>VAQISPQYPMFTVPLPIPPVKQPRLTVTNPVNGQEIWYYEVEIKPFTHQVYPDLGSADLVGYDGMSPGPTFQVPRGVETVVRFINNAEAPNSVHLHGSFSRAAFDGWAEDITEPGSFKDYYYPNRQSARTLWYHDHAMHITAENAYRGQAGLYMLTDPAEDALNLPSGYGEFDIPMILTSKQYTANGNLVTTNGELNSFWGDVIHVNGQPWPFKNVEPRKYRFRFLDAAVSRSFGLYFADTDAIDTRLPFKVIASDSGLLEHPADTSLLYISMAERYEVVFDFSDYAGKTIELRNLGGSIGGIGTDTDYDNTDKVMRFVVADDTTQPDTSVVPANLRDVPFPSPTTNTPRQFRFGRTGPTWTINGVAFADVQNRLLANVPVGTVERWELINAGNGATHPIHIHLVDFKVISRTSGNNARTVMPYESGLKDVVWLGRRETVVVEAHYAPFPGVYMFHCHNLIHEDHDMMAAFNATVLPDYGYNATVFVDPMEELWQARPYELGEFQAQSGQFSVQAVTERIQTMAEYRPYAAADE[2x]

Bilirubin oxidase (MvBOx; EC 1.3.3.5) from the ascomycete plant pathogen Myrothecium verrucaria (Albifimbria verrucaria) is a member of the blue multicopper oxidase family (MCO). MCOs are capable of oxidizing various organic and/or inorganic substrates and reducing oxygen to water without release of reactive oxygen species. MvBOx, composed of 534 amino acid residues, consists of three cupredoxin-like domains with four copper ions forming two active sites. T1Cu is connected with the trinuclear cluster (TNC), composed of one type II (T2Cu) and two type III (T3Cu) copper ions, via a conserved His–Cys–His motif (serving as electron transfer path).

Trp396 was mutated to alanine (MvBOxW396A) in order to enable direct solvent access to His398, to phenylalanine (MvBOxW396F) in order to introduce an aromatic residue not capable of crosslink formation, and to aspartic acid (MvBOxW396D) in order to disrupt this site by introducing negative charge. In the structure W396A:FECN, a ferricyanide ion is bound in the same site but shifted towards the T1Cu site, with the closest observed distance to T1Cu now being 9.2 Å, and interacting through a water molecule with His398 which coordinates T1Cu. It still interacts with the main chain nitrogen atoms of Asn394 and Gly395 but now through two of its cyanide moieties. It also interacts with the main chain nitrogen atom of Ala396 and with Arg356 via two adjacent cyanide moieties. The main difference in binding of ferricyanide between MvBOxWT and MvBOxW396A lies in the fact that the replacement of Trp by Ala allows ferricyanide to bind closer to T1Cu. Ferricyanide in the W396A mutant interacts with T1Cu-coordinating His398 through a water molecule, possibly mediating electron transfer. Ferricyanide (product) binds in the same site in both MvBOxWT and MvBOxW396A, although in two different poses. And even if Trp396 forms a part of the ferricyanide binding site in the wild type, it is not necessary for its binding. Although the adduct is probably involved in electron transfer in MvBOxWT, its presence is not crucial in the case of ferrocyanide oxidation as electron transfer can be realized using another path, possibly via the protein main chain of the loop forming OS1 (residues 394–398) or via water molecule in the case of W396A:FECN. The W396A mutant binds bilirubin with a lower affinity when compared to the wild type.>[2x]MGSSHHHHHHSQDPMSLNLVSEQLLAANGLKHQDLFAILGQLAERRLDYGDLYFQSSYHESWVLEDRIIKDGSYNIDQGVGVRAISGEKTGFAYADQISLLALEQSAQAARTIVRDSGDGKVQTLGAVEHSPLYTSVDPLQSMSREEKLDILRRVDKVAREADKRVQEVTASLSGVYELILVAATDGTLAADVRPLVRLSVSVLVEEDGKRERGASGGGGRFGYEFFLADLDGEVRADAWAKEAVRMALVNLSAVAAPAGTMPVVLGAGWPGVLLAEAVGHGLEGDFNRRGTSVFSGQVGELVASELCTVVDDGTMVDRRGSVAIDDEGTPGQYNVLIENGILKGYMQDKLNARLMGMTPTGNGRRESYAHLPMPRMTNTYMLPGKSTPQEIIESVEYGIYAPNFGGGQVDITSDKFVFSTS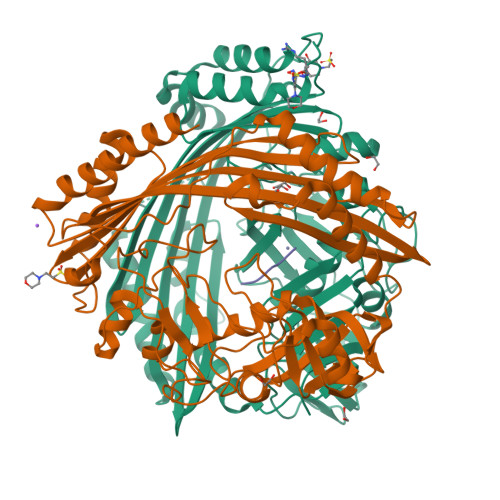EAYLIENGKVTKPVKGATLIGSGIETMQQISMVGNDLKLDNGVGVCGKEGQSLPVGVGQPTLKVDNLTVGGTA;>[2x]MALAMKVISQVEAQRKILEEAVSTALELASGKSDGAEVAVSKTTGISVSTRYGEVENVEFNSDGALGITVYHQNRKGSASSTDLSPQAIARTVQAALDIARYTSPDPCAGVADKELLAFDAPDLDLFHPAEVSPDEAIELAARAEQAALQADKRITNTEGGSFNSHYGVKVFGNSHGMLQGYCSTRHSLSSCVIAEENGDMERDYAYTIGRAMSDLQTPEWVGADCARRTLSRLSPRKLSTMKAPVIFANEVATGLFGHLVGAIAGGSVYRKSTFLLDSLGKQILPDWLTIEEHPHLLKGLASTPFDSEGVRTERRDIIKDGILTQWLLTSYSARKLGLKSTGHAGGIHNWRIAGQGLSFEQMLKEMGTGLVVTELMGQGVSAITGDYSRGAAGFWVENGEIQYPVSEITIAGNLKDMWRNIVTVGNDIETRSNIQCGSVLLPEMKIAGQ;>AAAAA[2x]> SQVSPTRMNLLQRRGQLRLAQKGVDLLKKKRDALVAEFFGLVREAMEARKALDQAAKE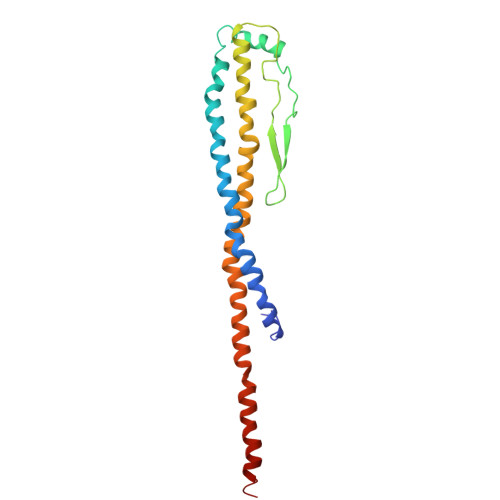AYAALLLAQAFDGPEVVAGAALGVPPLEGVEAEVENVWGSKVPRLKATFPDGALLSPVGTPAYTLEASRAFRRYAEALIRVANTETRLKKIGEEIKKTTRRVNALEQVVIPGIRAQIRFIQQVLEQREREDTFRLKRIKGKIEAREAEEEGG> PISSTP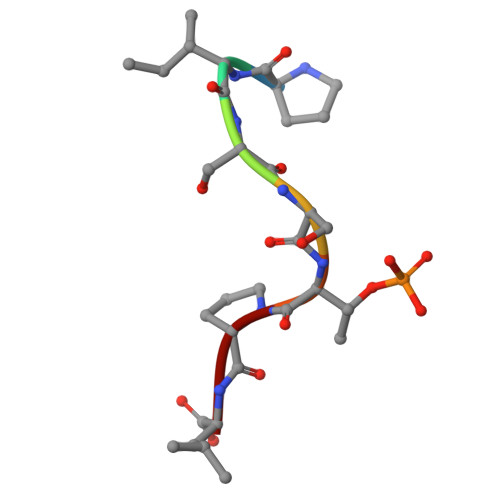L> TTNKPIVLSTWNFGLHANVEAWKVLSKGGKALDAVEKGVRLVEDDPTERSVGYGGRPDRDGRVTLDACIMDENYNIGSVAC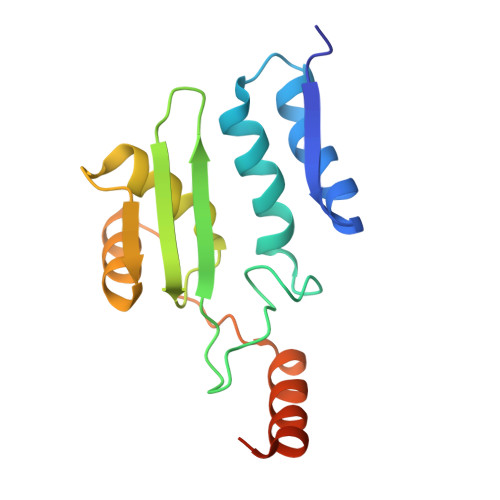MEHIKNPISVARAVMEKTPHVMLVGDGALEFALSQGFKKENLLTAESEKEWKEWLKTSQYKPIVNIENHD>DRWIRPRGAFGGLPSLKSSFVLSESTVPGTNETVKTFLPYGSVINYYGYVKPGQAPDGLVDGNKKAYYLYVWIPAVIAEMGVRMISPTGEIGEPGDGDLVSDAFKAATPEEKSMPHWFDTWIRVERMSAIMPDQIAKAAKAKPVQKLDDDDDGDDTYKEERHNKY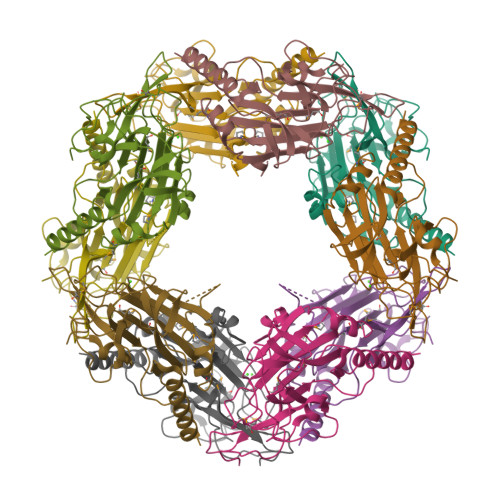NSLTRIKIPNPPKSFDDLKNIDTKKLLVRGLYRISFTTYKPGEVKGSFVASVGLLFPPGIPGVSPLIHSNPEELQKQAIAAEESLKKAASDATK[5x]Centromeric chromatin in fission yeast is distinguished by the presence of nucleosomes containing the histone H3 variant Cnp1CENP-A. Cell cycle–specific deposition of Cnp1 requires the Mis16–Mis18–Mis19 complex, which is thought to direct recruitment of Scm3-chaperoned Cnp1/histone H4 dimers to DNA. Mis16 is a homologue of the human WD40-repeat protein RbAp46/48, a well-known histone chaperone found in a variety of chromatin-associated complexes, whereas Mis19 seems to form a bridge between Mis16 and Mis18 with its N terminus binding Mis18 and C terminus binding Mis16. Current structural and biochemical data suggest a model in which Mis18 provides the principal link to the centromere, whereas Mis16 is responsible for recruitment of the Scm3–Cnp1–H4 complex, which allows Cnp1–H4 dimers to be inserted into chromatin as a prelude to complete nucleosome assembly. As expected, Mis16 adopts a β-propeller fold, consisting of 7 WD-40 repeats, with an extended N-terminal α-helix that forms part of the histone interaction pocket.

We identified a N-terminal truncation of Mis19 (residues 51–112, Mis19C) that was capable of interaction with Mis16. The crystal structure of Mis16–Mis19C was solved at 2.0 Å by molecular replacement using Mis16 as a search model. Mis19C forms an extended tether, which is able to bind two molecules of Mis16, one at each end. Residues 56–63 form a β-strand that continues β-propeller 7 of Mis16 and stabilises an extended loop from 107 to 116, which is disordered in the Mis16 structure alone. Mis19 then loops across the C-terminal face of the Mis16 disc and then forms a helix (α1, residues 79–97) running diagonally across the edge of the H4-binding pocket. This helix leads into a short loop, and finally into the C-terminal helix (α2, residues 99–111), which sits in the H4-binding site of a symmetry-related Mis16 molecule. Analysis of the structure shows three main contacts between Mis16 and Mis19. The first (site A) is formed by the Mis19 β-strand and proximal loop. The third (site C) comprises the C-terminal helix that binds to the same binding pocket of Mis16 as H4α1. In our Mis16–Mis19C crystal structure, two Mis19 molecules bind two Mis16 molecules in trans, with sites A and B binding one Mis16, whereas site C binds the second molecule.

>GSEEVVQDAPLENNELNAEIDLQKTIQEEYKLWKQNVPFLYDLVITHALEWPSLTIQWLPDKKTIPGTDYSIQRLILGTHTSGNDQNYLQIASVQLPNFDEDTTEFTPSTIRRAQATGSYTIEISQKIPHDGDVNRARYMPQKPEIIATMGEGGNAYIFDTTCHDALTTGEALPQAVLKGHTAEGFGLCWNPNLPGNLATGAEDQVICLWDVQTQSFTSSETKVISPIAKYHRHTDIVNDVQFHPQHEALLASVSDDCTLQIHDTRLNPEEEAPKVIQAHSKAINAVAINPFNDYLLATASADKTVALWDLRNPYQRLHTLEGHEDEVYGLEWSPHDEPILASSSTDRRVCIWDLEKIGEEQTPEDAEDGSPELLFMHGGHTNRISEFSWCPNERWVVGSLADDNILQIWSPSRVIWGRDHVQVSPRDLE[2x];>[2x]PRVYETELLVLRFREFGVKDNHNHPINLHSLRSKSLIRAQGKKLDLHNRVFLRRNVRAVKM> 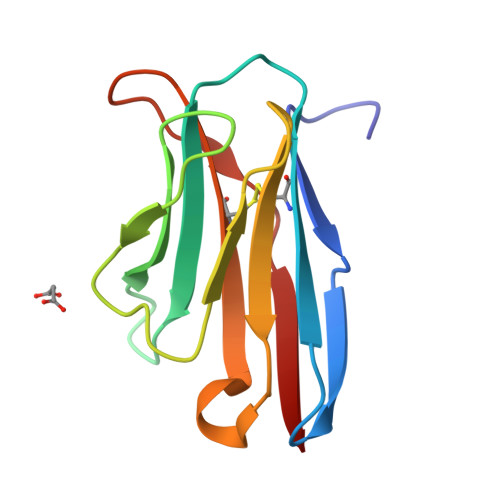ILEAAVTQSPRNKVAVTGEKVTLSCQQTNNHNNMYWYRQDTGHGLRLIHYSYGVGNTEKGDIPDGYEASRPSQEQFSLILELATPSQTTVYFCASGGGGTLYFGAGTRLSVL>TAELKICRVNRNSGSCLGGDEIFLLCDKVQKEDIEVYFTGPGWEARGSFSQADVHRQVAIVFRTPPYADPSLQAPVRV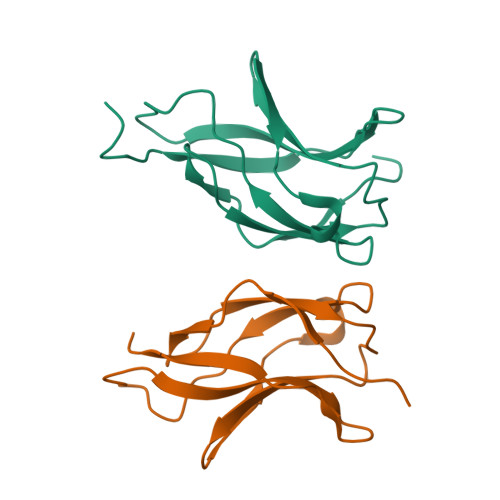SMQLRRPSDRELSEPMEFQYLPDTDDRHRIEEKRKR[2x]>[4x]MTIEYLKKASLTSKSDASDVQETVR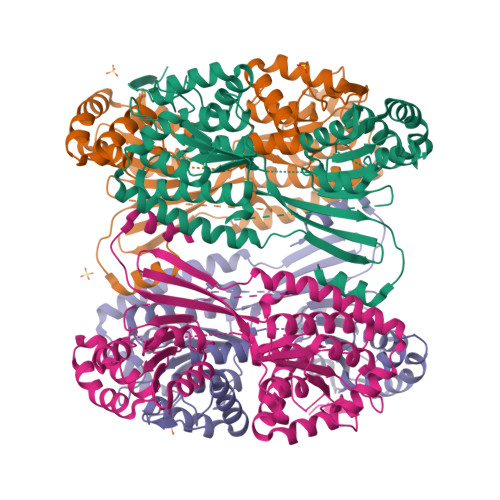AILADIEAGGDQVALDYAAKFDRYEGSIILSPEEIEAACAKVPEKLKADIRFAHDNVRRFAETQKATLTDVELEVVPGVITGQKAIPVDAAGCYVPGGRYSHIASAIMTVTTAKVAGCKHIMACSPPRPGVGVAPAIVYAAHICGADTIMAIGGVQGVASMAFGLFGLPKAKILVGPGNQFVAEAKRMLFGRVGIDMIAGPTDSLILADRTADPHIVTTDLVSQAEHGYNSPVWLVTDDRALAEKVIEMIPSYIADLPEVNRDNAAAAWRDYAEVILCADREEMAATSDRYAPEHLTVMAEDLDWWLDRLSCYGSLFLGEESTVSYGDKAAGTNHVLPTSGAASYTGGLSVHKYMKIVTWQRGTREGYKPVAEATARIARLE>KKRLTESQFQEAIQGLEVGQQTIEIARGVLVDGKPQATFATSLGLTRGAVSQAVHRVWAAFEDKNLPEGYARVTAVLPEHQAYIVRKWEADAKKKQ[2x];>[6x]KKRLTESQFQEAIQGLEVGQQTIEIARGVLVDGK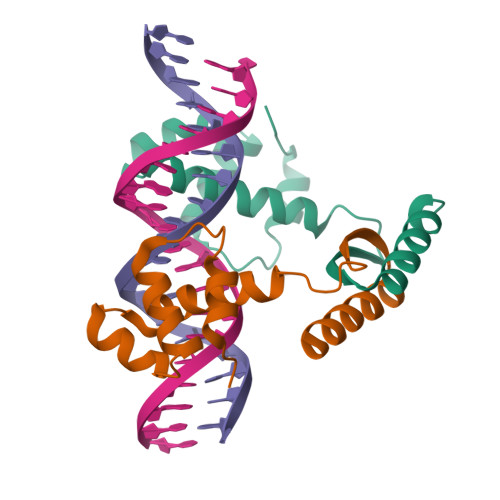PQATFATSLGLTRGAVSQAVHRVWAAFEDKN2-fluoranyl-6-methoxy-4-[4-methyl-5-[4-(4-propan-2-ylpiperazin-1-yl)phenyl]pyridin-3-yl]benzamide | C27 H31 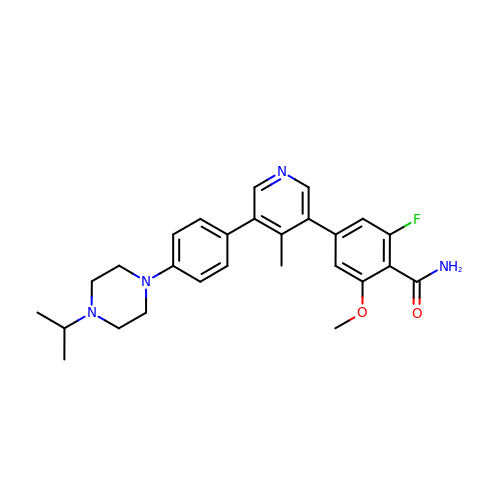F N4 O2 | RIWTUJFFSTVYPW-UHFFFAOYSA-N> MEAKAIAR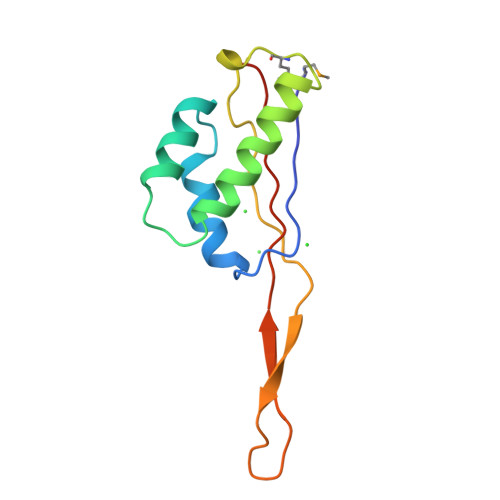YVRISPRKVRLVVDLIRGKSLEEARNILRYTNKRGAYFVAKVLESAAANAVNNHDMLEDRLYVKAAYVDEGPALKRVLPRARGRADIIKKRTSHITVILGEKHGK>MSVVGTPKSAEQIQQEWDTNPRWKDVTRTYSAEDVVALQGSVVEEHTLARRGAEVLWEQLHDLEWVNALGALTGNMAVQQVRAGLKAIYLSGWQVAGDANLSGHTYPDQSLYPANSVPQVVRRINNALQRADQIAKIEGDTSVENWLAPIVADGEAGFGGALNVYELQKALIAAGVAGSHWEDQLASEKKCGHLGGKVLIPTQQHIRTLTSARLAADVADVPTVVIARTDAEAATLITS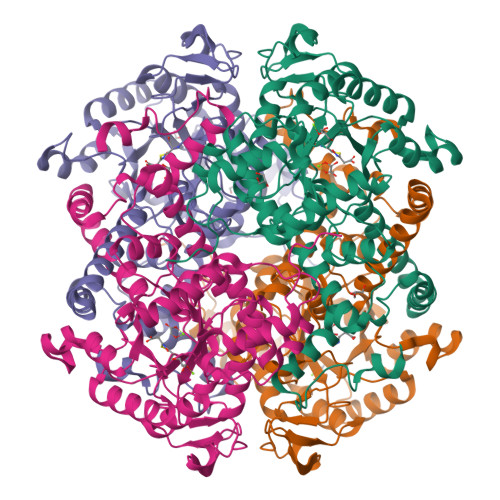DVDERDQPFITGERTREGFYRTKNGIEPCIARAKAYAPFADLIWMETGTPDLEAARQFSEAVKAEYPDQMLAYNCSPSFNWKKHLDDATIAKFQKELAAMGFKFQFITLAGFHALNYSMFDLAYGYAQNQMSAYVELQEREFAAEERGYTATKHQREVGAGYFDRIATTVDPNSSTTALTGSTEEGQFH[4x]One of these energy-consuming enzymes is the conserved huge AAA+-type ATPase Rea1 (also known as Mdn1), which is composed of a hexameric AAA+-ATPase domain, followed by a long tail consisting of an α-helical linker region, a flexible aspartate/glutamate (D/E)-rich domain and a C-terminal metal-ion-dependent adhesion site (MIDAS) homologous to the inserted (I) domain within the α-subunits (αI) of integrins that mediate ligand recognition. The conserved interaction between the C-terminal Rea1-MIDAS and the Rsa4-UBL (ubiquitin-like domain) or Ytm1-UBL is essential for assembly of the 60S pre-ribosome in a reaction mediated by the Rea1 ATPase upon ATP hydrolysis that leads to the removal of Ytm1 and Rsa4 from distinct pre-60S intermediates. In this study, we report crystal structures of the Chaetomium thermophilum (Ct) Rea1-MIDAS, both alone and in complex with its pre-ribosomal substrates, the CtYtm1- or CtRsa4-UBL domains. Besides displaying the typical MIDAS fold known for integrins, the CtRea1-MIDAS crystal structures reveal evolutionary conserved Rea1 specific structural elements.

However, due to the low yield and solubility of this construct, we switched to the thermostable Rea1-MIDAS from C. thermophilum (Ct). This construct (CtRea1-MIDAS) carries a ~105 residue-long N-terminal extension, which is absent from integrin MIDAS domains but is known to contribute to Ytm1 and Rsa4 binding both in yeast and human. We were able to purify the CtRea1-MIDAS construct in sufficient amount to allow us to obtain crystals and determine its crystal structure at 2.3 Å (for data collection and refinement statistics). However, the CtRea1-MIDAS contains three additional conserved structural elements (termed elements I, II and III) that are not present in integrin-MIDAS domains. The first half of the Rea1-specific N-terminal extension contains a long α-helix (element I), which wraps around the MIDAS domain core. Although this part of the N-terminal extension (amino acids 4693–4732) has a low-sequence conservation, it contains an invariant tryptophan residue in the first part of the helix (W4710 in C. thermophilum and W4633 in S. cerevisiae), which packs between helices α3 and α4 and most likely anchors the N-terminal helix in place. The second Rea1-specific MIDAS element (II, termed loop) forms a 45 amino-acid-long disordered loop (amino acids 4733–4777) opposite the critical DxSxS motif. The third MIDAS element (III) is located in the C-terminal region preceding the last α-helix of the classical α/β Rossmann fold. Rigid body fitting of the CtRea1-MIDAS into the density map of S. pombe Rea1 unambiguously identified the Rea1-MIDAS loop attached to the Rea1-AAA+ inner pore ring.

> MEEDLEDEQIKEASSQLLATHISDEQLKRPLRDYGEALEMWSTFQTKTQALSQSLSSQLRLILTPTQSTKLSGAFRTGKRLNIKKIIPYIASSYKRDKIWMRRAIPSKRAYQILLCVDDSSSMSDDNRSTAGNLALESLVMVARALTVLEAGQIGVMGFGTDVFVAHALTDPPFTSQDAGARVLQQFTFRQDSTDMVLLLRRTIDHFREARLIQASSSRGGEDLWQLALILSDGLVQSRDHARLRPLLREAMEQRVMVVFIVMDDARSRKGHSVLELKEARFGPDGVPVIHRYLDSFPFPYYLIVHHLEDLPGALAALLRTWFAEVNSGSHHHHHH>[2x]MERPQLDSMSQDLSEAL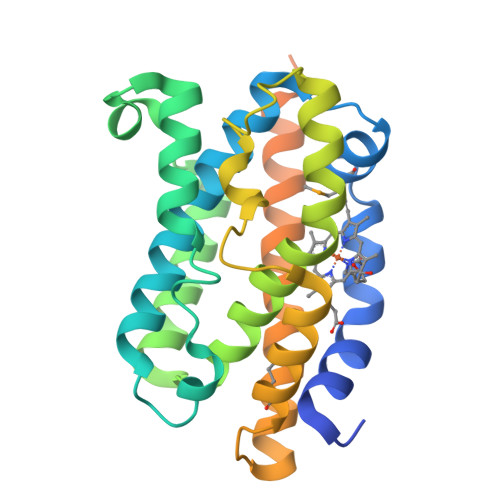KEATKEVHIRAENSEFMRNFQKGQVSREGFKLVTASLYHIYTALEEEIERNKQNPVYAPLYFPEELHRRAALEQDLAFWYGPHWQEAIPYTPATQHYVKRLHEVGGTHPELLVAHAYTRYLGDLSGGQVLKKIAQKALALPSSGEGLASFTFPSIDNPTKFKQLYRARMNTLELTPEVKHRVTEEAKTAFLLNIELFEELQALLTEEHKDQSPSQTEFLRQRPASLVQDTTSAETPRGKSQISTSSSQTP>GEVPIGFDTDELSFDMSLVLLTGDMQTKASDPNYTYATTEELTIQNCHVAVFDKDGKRIYFKNFYSKDLGEMKTIGNLSGYELQLEGVR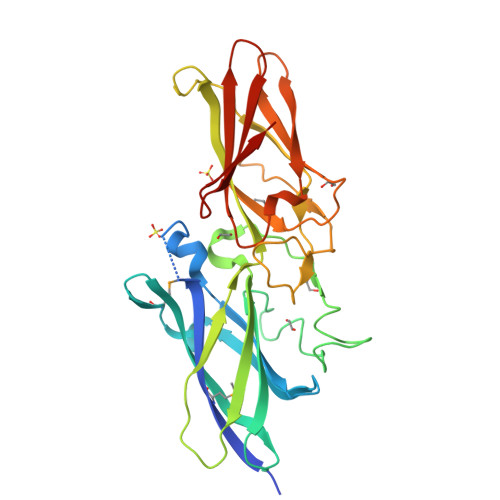TFGKEDKKVSVLVVANANNANNSPFDNLTTYDGVDNSYTAKTIAKGPVTASLLVKIGKSETTLKYNQDNAPVTVSLIQLSAKIEYTGVYKKENGELLEGFSLTKVAGLNASSKITIFNTSAVENGAFSDLAYPTTKPVTFYTYEISDAFKEVILSVQSGVEPKEYPFPANKFIKGNYYRIKGLKSSTEIEWVLENVEDKEVTLDPFE[2x]> MEIIHLSEIDSTNDYAKELAKEGKRNFIVLADKQNNGKGRWGRVWYSDEGGLY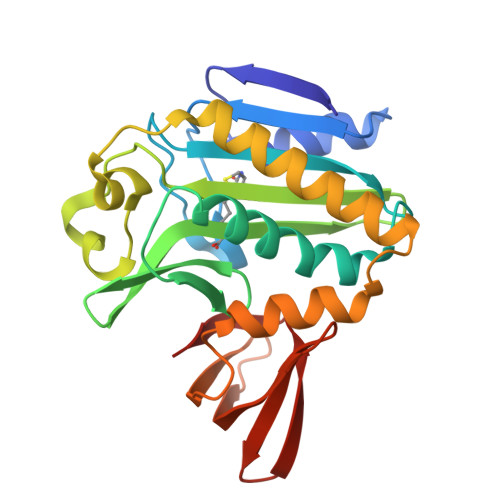FSMVLDSKLYNPKVINLLVPICIIEVLKNYVDKELGLKFPNDIMVKVNDNYKKLGGILTELTDDYMIIGIGINVNNQIRNEIREIAISLKEITGKELDKVEILSNFLKTFESYLEKLKNKEIDDYEILKKYKKYSITIGKQVKILLSNNEIITGKVYDIDFDGIVLGTEKGIERIPSGICIHVR>[2x]MRDKTMIKQRTLKRIVQATGVGL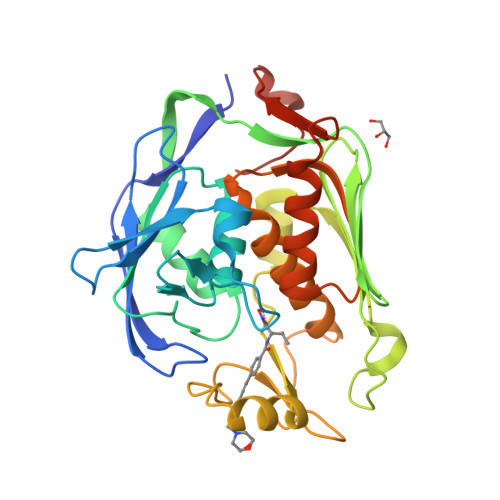HTGKKVTLTMRPAPANTGVIYRRTDLNPPVDFPADAKSVRDTMLCTCLVNEHDVRISTVEHLNAALAGLGIDNIIIEVNAPEVPIMDGSASPFVYLLLDAGIEELNSAKKFLRLKETVRVEDGDKWAELSPFNGFRLDFTIDFNHPAIDSSTQRYRLDFSADSFVRQISRARTFGFMRDIEYLQSRGLCLGGSFDCAIVVDDYRVLNEDGLRFEDEFVRHKMLDAIGDLFMCGHNIIGAFTAYKSGHALNNKLLQAVLAKQEAWEFVTFQDEAEMPLAFKAPSTVLAY> GPGSMSDTVIERHADTAALVAAAGDRLVDAISSAIGERGQATIVLTGGGTGIGLLKRVRERSGEIDWSKVHIYWGDERFVPQ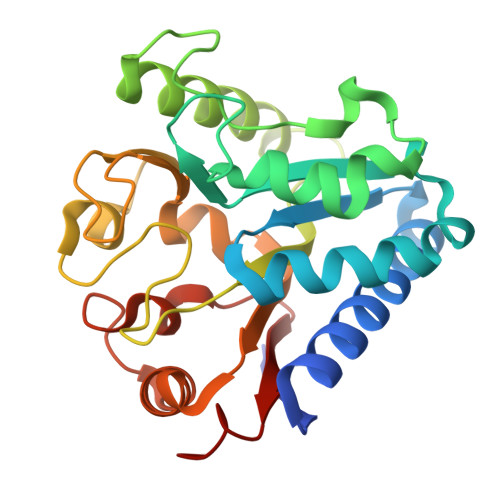DDDERNDKQAREALLDHIGIPPVNVHAMAASDGEFGDDLEAAAAGYAQLLSANFDSSVPGFDVHLLGMGGEGHVNSLFPDTDAVRETERLVVGVSDSPKPPPRRITLTLPAVQNSREVWLVVSGEAKADAVAAAVGGADPVDIPAAGAVGRERTVWLVDEAAAAKL> MAAGSITTLPALPEDGGSGAFPPGHFKDPKRLYCKNGGFFLRIHPDGRVDGVREKSDPHIKLQLQAEERGVVSIKGVSANRYLAMKEDGRLLASKSVTDECFFFERLESNNYNTYRSRKYTSWYVALKRTGQYK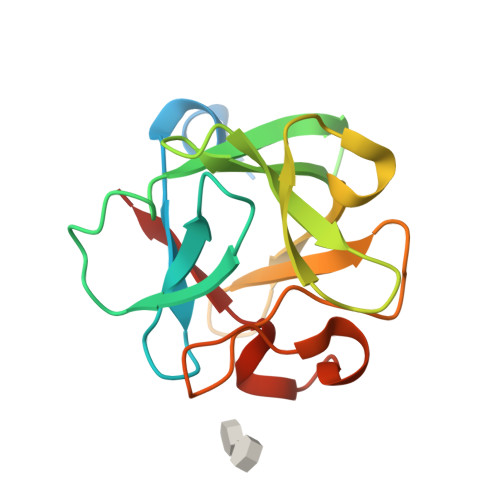LGSKTGPGQKAILFLPMSAKS>MENDPNLFVALYDFVASGDNTLSITKGEKLRVLGYNHNGEWCEAQTKN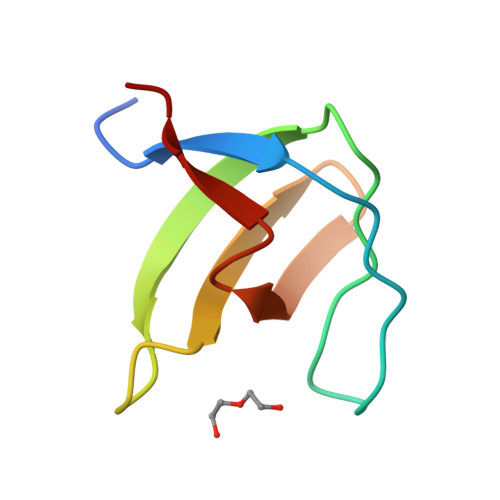GQGWVPSNYITPVNS[2x]Bacteriophage (phage) vB_EcoM_CBA120, discovered by Kutter and colleagues, is a member of the recently defined Kuttervirus genus of contractile tailed phages belonging to the Ackermannviridae family. Each TSP recognizes a different lipopolysaccharide on the membrane of a different bacterial host. The 335 N-terminal residues of TSP4 promote the assembly of the TSP complex and anchor it to the tail baseplate.

Herewith we refer to this construct as TSP4-N490. This protein degraded within the period of crystal growth in poly ethylene glycol 8000 solution, yielding a structure that lacked the XD3 domain. Although the exact cleavage site is unknown, 250 residues could be traced in the electron density map. In the following discussion, this structure is named TSP4-N250 to distinguish it from TSP4-N253, one of the protein variants that was designed to identify the TSP4-N domain interactions with partner TSPs by AUC. The TSP4-N250 structure was determined by molecular replacement. Indeed, the crystal structure of TSP4-N250, lacking the XD3 domain, shows three XD2 domains packed together, consistent with the arrangement necessary for promoting trimeric protein–protein interaction. In contrast, the three linkers are conformationally disordered in the crystal structure of TSP4-N250, and bring the three XD2 domains together to interact along the crystallographic threefold symmetry axis. In contrast, the analogous binding surface of the closely associated XD2 trimer as seen in the TSP4-N250 structure, is more neutral, with three lysine residues forming a positively charged patch in the center of the solvent exposed surface. The TSP4 XD2 trimer binding surface, as seen in the TSP4-N250 crystal structure, exhibits positively charged residues at the center and negatively charged residues at the rim. Nevertheless, the TSP4-N250 crystal structure shows that the TSP4 XD2 domain can form a closely packed trimer and the flexible linkers can adjust the relative orientations between the globular trimeric domains.

> MANKPTQPLFPLGLETSESSNIKGFNNSGTIEHSPGAVMTFPEDTEVTGLPSSVRYNPDSDEFEGYYENGGWLSLGGGGIRWETLPHAPSSNLLEGRGYLINNTTGTSTVVLPSPTRIGDSVTICDAYGKFATYPLTVSPSGNNLYGSTEDMAITTDNVSATFTWSGPEQGWVITSGVGLGQGRVYSREIFTQILASETSAVTLNTPPTIVDVYADGKRLAESKYSLDGNVITFSPSLPASTELQVIEYT>MSLGVTQ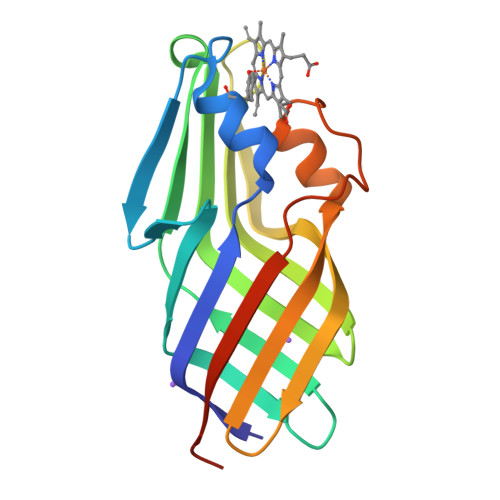ASAQWGVKASFQNYIRGSIANGSWTLNGVGFDNQQFQFSGNSGAVDAENKTGSINFPGSIHFTGAGGILDMQIANIEISFNGNSGELIADVVSSDMDGNSTNYGRTVVGTLNFSALNVSATEASGSASVSLSQSGSQAFADFYTPGTQLDPISFSATLGGLEHHHHHH[2x]[1-(4-oxidanylphenoxy)-1-phosphono-ethyl]phosphonic acid | C8 H12 O8 P2 | 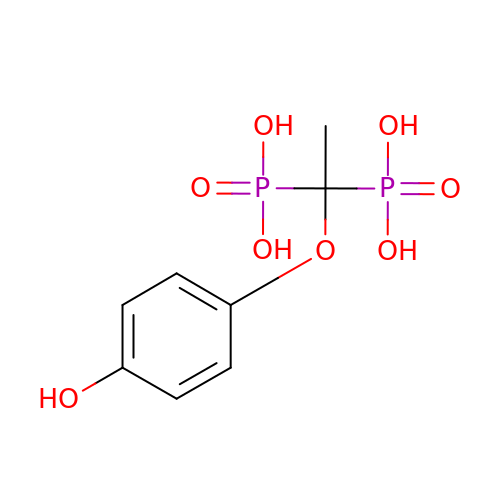JKOCAAWWDVHWKB-UHFFFAOYSA-N6-[(5-cyclopropyl-1~{H}-pyrazol-3-yl)amino]-2-[4-[(3-methyl-4-oxidanyl-phenyl)methyl]piperazin-1-yl]-~{N}-prop-2-ynyl-pyrimidine-4-carboxamide 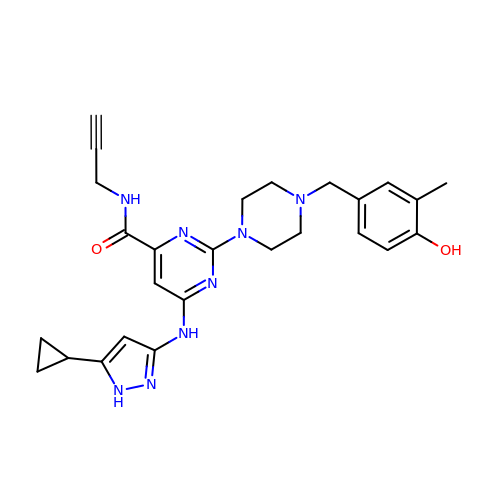| C26 H30 N8 O2 | VCHMYWXCLCHLBE-UHFFFAOYSA-N5-methoxy-1H-indole | C9 H9 N O | 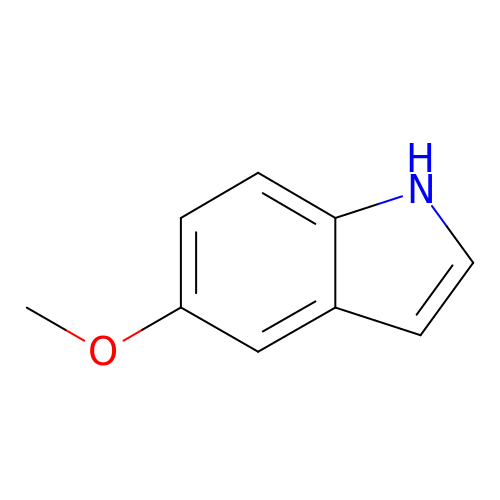DWAQDRSOVMLGRQ-UHFFFAOYSA-N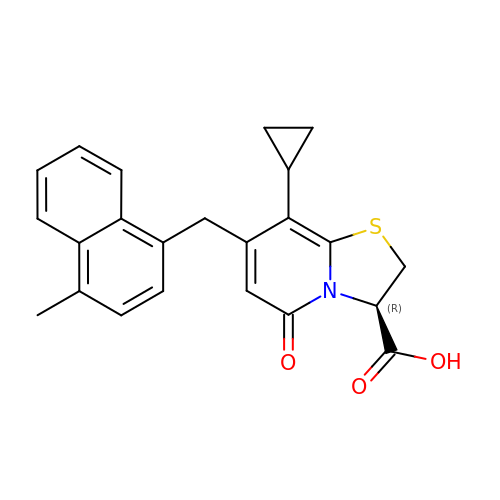(3~{R})-8-cyclopropyl-7-[(4-methylnaphthalen-1-yl)methyl]-5-oxidanylidene-2,3-dihydro-[1,3]thiazolo[3,2-a]pyridine-3-carboxylic acid | C23 H21 N O3 S | XQPUCYFOBBJYCO-IBGZPJMESA-N>[2x]MAAVSEVAVDGVVFPPVARPPGSGRSHFLAGAGVRGMEIGGNFIKFTAIGVYLEEGAAVSALAKKWAGKSADELAAD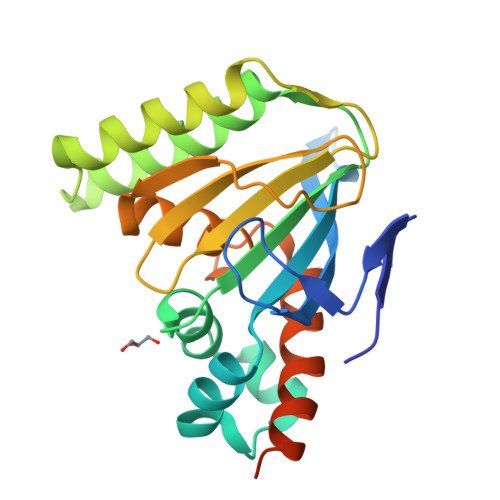AAFFRDVVTGDFEKFTRVTMILPLTGEQYSGKVTENCVAYWKAVGVYTDAEGAAVDKFKEAFKPETFPPGASILFTHSPAGVLTVAFSKDSSVPESGGVAIDNKPLCEAVLESIIGEHGVSPAAKLSVAARVSELLKEASPAGGAPQAAAEPAVPVSAEF> MSPQDDLIVWLRGDRAGLGPFSAD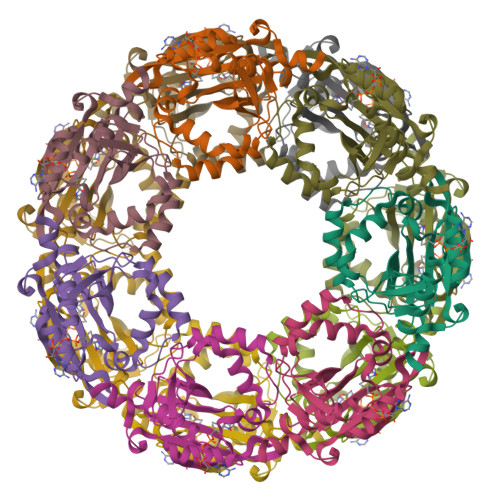LVDQYWRWEQDPSVLIGYGRQTPDSLENRREGYGHQARGTDDQLRFTVYDLTGQDPVPVGTTAVLIDHHVRTGEFVIQLGAGHRGRGLGTEATRLTLDYAFHVSALACVHLAVLTPNTGAIAAYERAGFRRIGERRDSGFWLGRRVSETLMDAVPEDFPGPSVVRGFVEGGR> AQYEDGKQYTTLEKPVAGAPQVLEFFSFFCPHCYQFEEVLHISDNVKKKLPEGVKMTKYHVNFMGGDLGKDLTQAWAVAMALGVEDKVTVPLFEGVQKTQTIRSASDIRDVFINAGIKGEEYDAAWNSFVVKSLVAQQEKAAADVQLRGVPAMFVNGKYQLNPQGMDTSNMDVFVQQYADTVKYLSEKK

DsbA enzymes catalyze oxidative folding of proteins that are secreted into the periplasm of Gram‐negative bacteria, and they are indispensable for the virulence of human pathogens such as Vibrio cholerae and Escherichia coli. DsbA enzymes retain a conserved tertiary structure, comprising a classical thioredoxin (TRX) domain with an inserted α‐helical domain. The TRX domain contains a pair of redox‐active cysteine residues in a CXXC motif located adjacent to a conserved cis‐proline residue. These features contribute to a hydrophobic patch of residues located in a surface groove of DsbA that is required for substrate recognition.

To identify the structural details of the interaction between TC and DsbA, we solved the crystal structures of TC in complex with oxidized EcDsbA and VcDsbA using molecular replacement at resolutions of 1.79 Å and 1.74 Å, respectively. In the complex with EcDsbA, TC occupies the full length of the hydrophobic groove and buries 435 Å2 of solvent accessible surface area (SASA). It interacts with H32 in the active site and cis‐P151, both of which are highly conserved in DsbA enzymes and critical for disulfide catalysis. The interaction with the steroid core at the right‐hand side of the groove (proximal to the active site) is driven by hydrophobic interactions with F36, L40, M171, F174, P163 and L161. On the left‐hand side (distal to the active site), the negatively charged sulfonate group of TC forms a network of polar interactions with the side chain amide of Q160 and a series of water molecules, and its amide NH forms a hydrogen bond with the backbone amide of cis‐P151. Additional polar contacts are made to a symmetry related EcDsbA molecule through the amide carbonyl and hydroxyl groups of TC which point away from the hydrophobic groove, however no hydrophobic interactions are made to the symmetry related EcDsbA molecule and the solution HSQC NMR data are consistent with the binding mode determined by X‐ray crystallography with significant CSP located in the hydrophobic groove. The side chains of F174, T168 and M171in EcDsbA are oriented towards the active site, which narrows the right‐hand side of the hydrophobic groove forming a small hydrophobic pocket around TC, pushing TC further towards the left‐hand end of the groove where additional interactions are formed. The VcDsbA‐TC interface consists of three direct polar interactions to the backbone amide of Gly161 and the side chains of His32 and Tyr170, whereas the EcDsbA‐TC interface has two direct polar interactions to the backbone of Pro151 and the side chain of Gln160. Comparison of the crystal structure of TC bound to EcDsbA with previously reported co‐structures of EcDsbA in complex with diaryl ether 3 shows the steroid core of TC makes similar hydrophobic interactions to diaryl ether 3 in the hydrophobic groove.> RSPWPGPPPAPPGLPAGADCLNSFTAGVPGFVLDTNASVSNGATFLESPTVRRGWDCVRACCTTQNCNLALVELQPDRGEDAIAACFLINCLYEQNFVCKFAPREGFINYLTREVYRSYRQLRTQGFGGSGIPKAWAGIDLKVQPQEPLVLKDVENTDWRLLRGDTDVRVERKDPNQVELWGLKEGTYLFQLTVTSSDHPEDTANVTVTVLSTKQTEDYCLASNKVGRCRGSFPRWYYDPTEQICKSFVYGGCLGNKNNYLREEECILACRGVQGPSMERRHPVCSGTCQPTQFRCSNGCCIDSFLECDDTPNCPDASDEAACEKYTSGFDELQRIHFPSDKGHCVDLPDTGLCKESIPRWYYNPFSEHCARFTYGGCYGNKNNFEEEQQC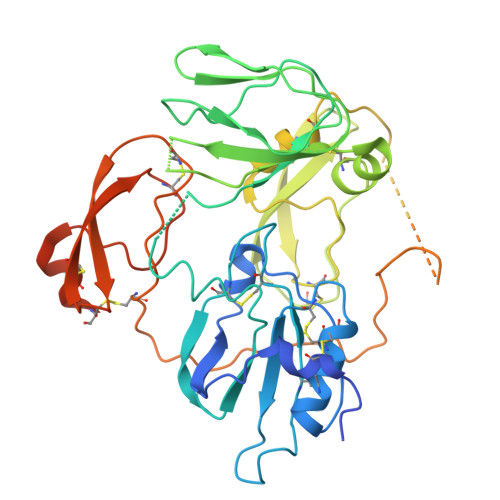LESCRGISKKDVFGLRREIPTRTGHHHHHH(2S)-3-{4-[4-(4-{[(2R)-2-hydroxy-3,3-dimethylbutyl]oxy}phenyl)heptan-4-yl]phenoxy}propane-1,2-diol 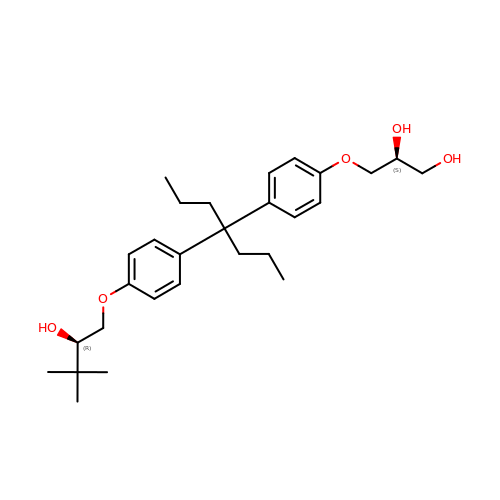| C28 H42 O5 | PJASVJJQJUYPCG-OZXSUGGESA-N> IVGGTSASAGDFPFIVSISRNGGPWCGGSLLNANTVLTAAHCVSGYAQSGFQIRAGSLSRTSGGITSSLSSVRVHPSYSGNNNDLAILKLSTSIPSGGNIGYARLAASGSDPVAGSSATVAGWGATSEGGSSTPVNLLKVTVPIVSRATCRA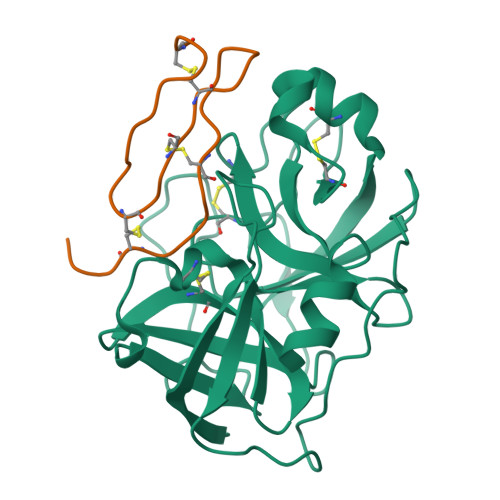QYGTSAITNQMFCAGVSSGGKDSCQGDSGGPIVDSSNTLIGAVSWGNGCARPNYSGVYASVGALRSFIDTYA;> ECTPGQTKKQDCNTCTCTPTGIWGCTRKACRTT>MSRLTGKNALVTGSSRGIGRATAVRLAREGALVAVHYASNEAAADETVAQIEREGGRAFPVRAELGVAGDVHELFLGLEQGLKERTGETTLDILVNNAAVTGVDGILPEDVTAEQLDRYYAVNAKAPFLLVQRAVRNMPDGGRIINISSGLTRCAVPEQVAYSMTKGALEQITLHMAKHLAPRGITVNSVAPGITDNGGAVFDIPEIVEQMAQSSAFKRVGEAGDVADVVTFIATDESRW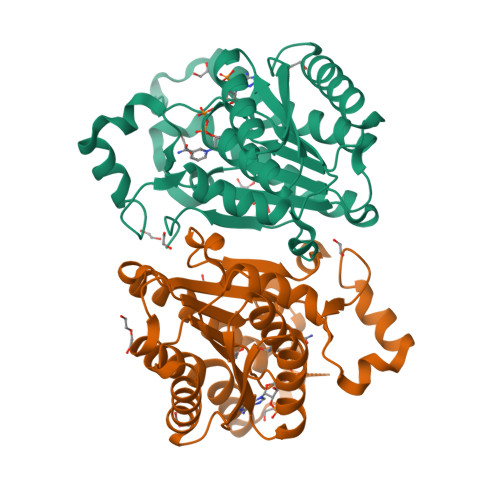ITGAFIDASGGTLLG[2x]Diterpene synthase VenA is responsible for assembling venezuelaene A with a unique 5-5-6-7 tetracyclic skeleton from geranylgeranyl pyrophosphate. VenA also demonstrates substrate promiscuity by accepting geranyl pyrophosphate and farnesyl pyrophosphate as alternative substrates. A promiscuous DTS VenA containing an atypical 115DSFVSD120 motif was characterized to catalyze the unique cyclization of geranylgeranyl pyrophosphate (GGPP, C20), giving rise to 1. The monomer of VenA holds a typical isoprenoid synthase α-fold comprised of twelve core α-helices and four additional short α-helices.

To provide structural basis for the substrate promiscuity and unique cyclization mode of VenA, we first sought to crystallize VenA in its substrate-free form. However, we did not obtain any crystals of the wild-type VenA (VenAWT) and supposed that the N-terminal flexible loop region (1-15 aa) might prevent the protein crystallization. Thus, the truncated form VenAΔ1-15 with the N-terminal fifteen amino acids removed was expressed and purified. Of note, the in vitro enzymatic assays indicated this modification did not affect the activity of VenA (we use “VenA” to stand for “VenAΔ1-15” unless otherwise specified). In the crystal structure, VenA is dimeric, which is consistent with the result of size exclusion chromatographic analysis, indicating that VenA forms a homodimer in solution as well. Helices B2, C, G1, G2, H, J, and α4 form the active site cavity, and helices A, B1, and C-terminal loop contribute to the dimer interface with a buried area of 2350.5 Å2. Similar to dimeric CotB2 and SVS-A2, the two monomers are organized in an antiparallel arrangement and each active site points away from the dimer interface. The PPi-Mg2+-bound and apo forms of VenA show slightly different conformations with a Cα root-mean-square deviation (RMSD) value of 0.327 Å. The obvious movements were found in C and H helices, which resulted from the binding of metal ions and PPi group by the catalytic motifs, including the atypical Asp-rich motif (115DSFVSD120) located on C-helix and NSE motif (256NDLLSWRKE264) on H-helix. The side chain of Tyr108 forms hydrogen bonds with the guanidine group of Arg344 in the apo form, but is rotated to the opposite direction in the holo form.

>[2x]EQIGGSVITDVDLTRRLLPGDGPGEFFLPPLPRLLPAGYHPDAARIEIASNGWVRRMLADCFDSEESLLFFLRQRNGIYGPLTVPYAEADRAQNIADWYQFVTVIDSFVSDEAALGADHAAAAETFAAVVADLREGGAGGPAASLYGRAAQDLWRRIAAGMSARQVDRLVAALEAFLRGCAEEIRSKLDKQVPHFEACMRVRVDSFGCEFLELLTEYAAEVDMSRAATEGLFDEVHHHGMRQLILVNDLLSWRKEYAQRDTMTTVRVLCEVEGLELQDAVDRLCALVEHHERAYITARDAVLAGPHGHREDVRAYLSGLDHLIGGSQEFEYLTPRYFGDGSVWDGSTSGWISLTASVARFRDAPAPAPSARPTRPLV>[2x]ISSCNGPCRDLNDCDGQLICIKGKCNDDPQVGTHICRGTTXSXQPGGCKPSGTLTCRGKSHPTY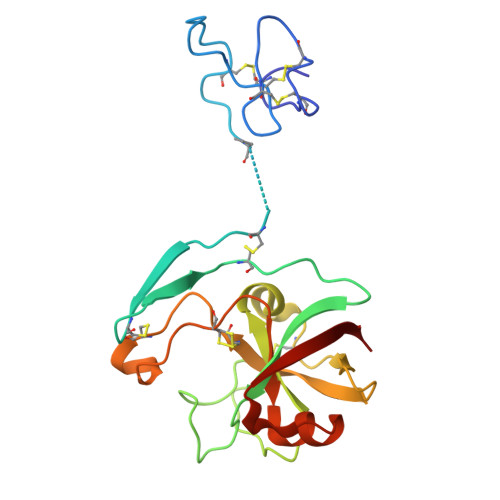DCSPPVTSSTPAKLTNNDFSEGGDDGGPSECDESYHNNNERIVALSTGWYNGGSRCGKMIRITASNGKSVSAKVVDECDSRHGCDKEHAGQPPCRNNIVDGSNAVWSALGLDKNVGVVDITWSMA>SNAEMSYELAQHGRSTLPRELAVYALEGPFFFAAAETFERVMGSIQETPQILILRLKWVPFMDITGIQTLEEMIQSFHKRGIKVLISGANSRVSQKLVKAGIVKLVGEQNVYPVFEGALSA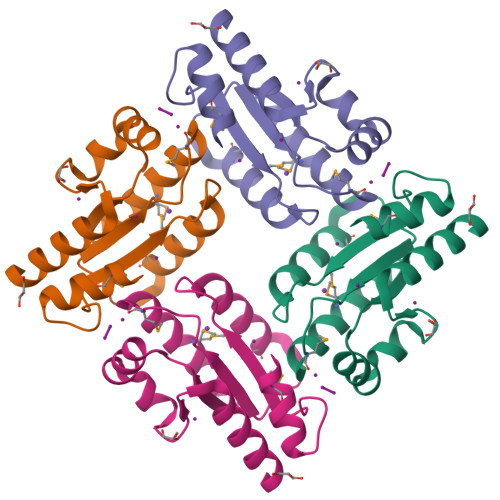ALTEIEAQP[2x]> QIASDVEAPPPAPAKVEKHSKKMEEGITVNKFKPKTPYVGRC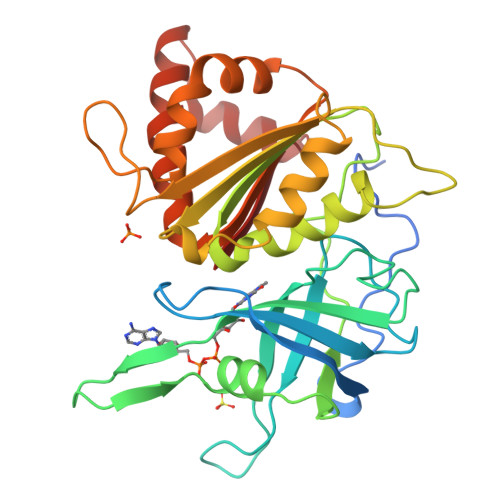LLNTKITGDDAPGETWHMVFSHEGEIPYREGQSVGVIPDGEDKNGKPHKLRLYSIASSALGDFGDAKSVSLCVKRLIYTNDAGETIKGVCSNFLCDLKPGAEVKLTGPVGKEMLMPKDPNATIIMLGTGTGIAPFRSFLWKMFFEKHDDYKFNGLAWLFLGVPTSSSLLYKEEFEKMKEKAPDNFRLDFAVSREQTNEKGEKMYIQTRMAQYAVELWEMLKKDNTYFYMCGLKGMEKGIDDIMVSLAAAEGIDWIEYKRQLKKAEQWNVLVY> MSSIVNKSGTRFAPKVRQRRAATGGTPTPKPRTPQLFIPESKEIEEDNSDNDKGVDENETAIVEKPSLVGERSLEGFTLTGTNGHDNEIGDEGPIDASTQNPKADVIEDNVTLKPAPLQTHRDQKVPRSSRLASLSKDNESRPSFKPSFLDSSSNSNGTARRLSTISNKLPKKIRLGSITENDMNLKTFKRHRVLGKPSSAKKPA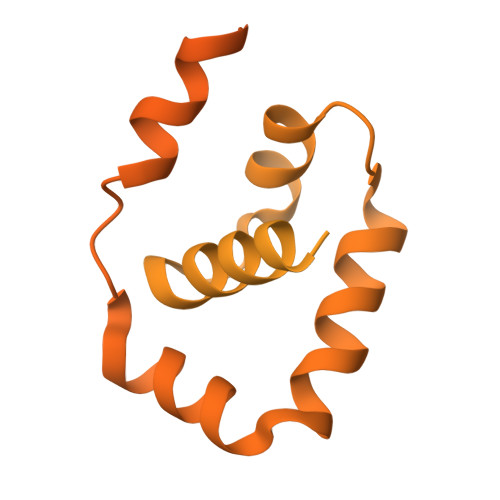GAHRISIVSKISPPTAMTDSLDRNEFSSETSTSREADENENYVISKVKDIPKKVRDGESAKYFIDEENFTMAELCKPNFPIGQISENFEKSKMAKKAKLEKRRHLRELRMRARQEFKPLHSLTKEEQEEEEEKRKEERDKLLNADIPESDRKAHTAIQLKLNPDGTMAIDEETMVVDRHKNASIENEYKEKVDENPFANLYNYGSYGRGSYTDPWTVEEMIKFYKALSMWGTDFNLISQLYPYRSRKQVKAKFVNEEKKRPILIELALRSKLPPNFDEYCCEIKKNIGTVADFNEKLIELQNEHKHHMKEIEEAKNTAKEEDQTAQRLNDANLNKKGSGGIMTNDLKVYRKTEVVLGTIDDLKRKKLKERNNDDNEDNEGSEEEPEIDQ> MTSFSRSQVLELERRFLRQKYLASAERAA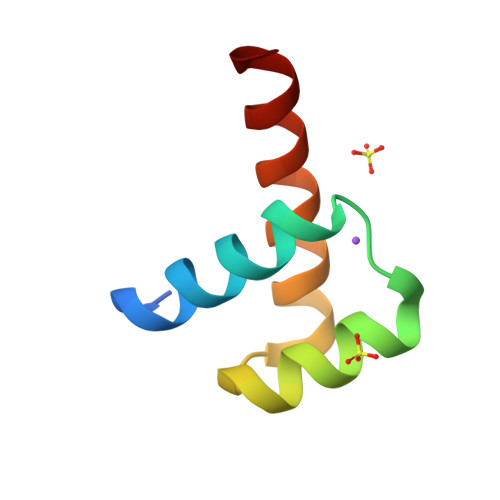LAKALRMTDAQVKTWFQNRRTKWRRQT> MYVRISGRIR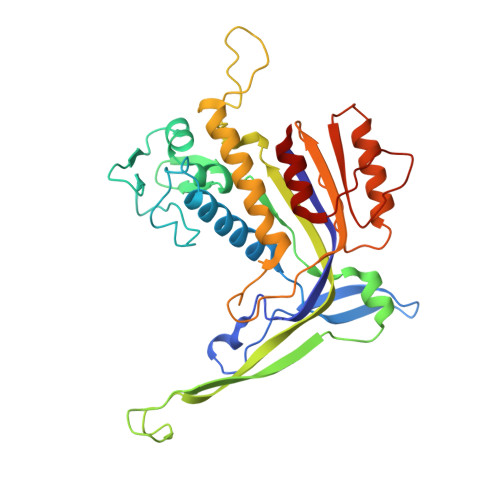LNAHSLNAQGGGGTNYIEITKTKVTVRTENGWTVVEVPAITGNMLKHWHFVGFVDYFKTTPYGVNLTERALRYNGTRFGQGETTATKANGATVQLNDEATIIKELADADVHGFLAPKTGRRRVSLVKASFILPTEDFIKEVEGERLITAIKHNRVDVDEKGAIGSSKEGTAQMLFSREYATGLYGFSIVLDLGLVGIPQGLPVKFEENQPRPNIVIDPNERKARIESALKALIPMLSGYIGANLARSFPVFKVEELVAIASEGPIPALVHGFYEDYIEANRSIIKNARALGFNIEVFTYNVDLGEDIEATKVSSVEELVANLVKMV> EGLEQLEAQTNFTKRELQVLYRGFKNECPSGVVNEDTFKQIYAQF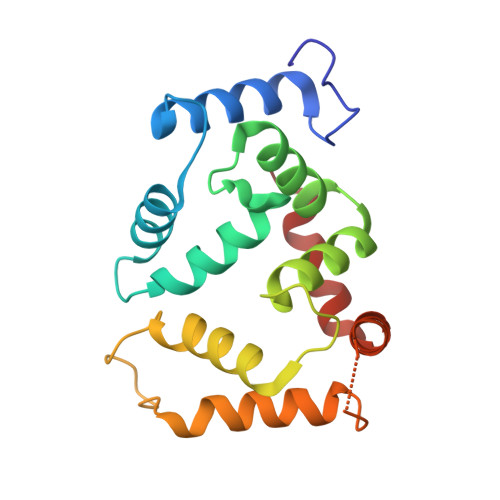FPHGDASTYAHYLFNAFDTTQTGSVKFEDFVTALSILLRGTVHEKLRWTFNLYDINKDGYINKEEMMDIVKAIYDMMGKYTYPVLKEDTPRQHVDVFFQKMDKNKDGIVTLDEFLESCQEDDNIMRSLQLFQNVM> HSLGKDDLRPSSPLLSVFGVLILTLLGFLVAATFAWNLLVLATILRVRTFHRVPHNLVASMAVSNVLVAALVMPLSLVHELSGRRWQLGRRLCQLWIACDVLCCTASIWNVTAIALDRYWSITRHMEYTLRTRKCVSNVMIALTWALSAVISLAPLLFGWGETYSEGSEECQVSREPSYAVFSTVGAFYLPLCVVLFVYWKIYKAAKFRVGSRKTNSVSPISEAVEVKDSAKQPQMVFTVRHATVTFQPEGDTWREQKEQRAALMVGILIGVFV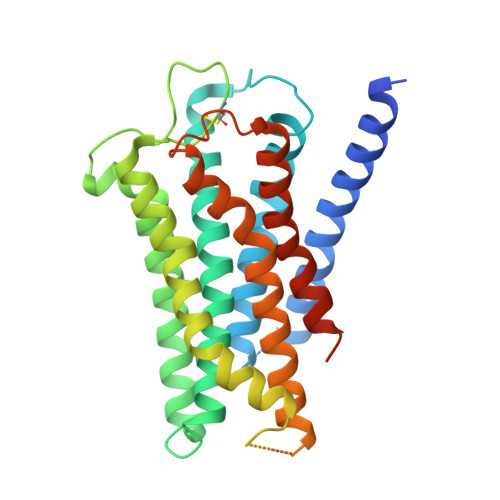LCWAPFFLTELISPLCSCDIPAIWKSIFLWLGYSNSFFNPLIYTAFNKNYNSAFKNFFSRQH>[16x]MVSLEKNDHLMLARQLPLKSVALILAGGRGTRLKDLTNKRAKPAVHFGGKFRIIDFALSNCINSGIRRMGVITQYQSHTLVQHIQRGWSFFNEEMNEFVDLLPAQQRMKGENWYRGTADAVTQNLDIIRRYKAEYVVILAGDHIYKQDYSRMLIDHVEKGARCTVACMPVPIEEASAFGVMAVDE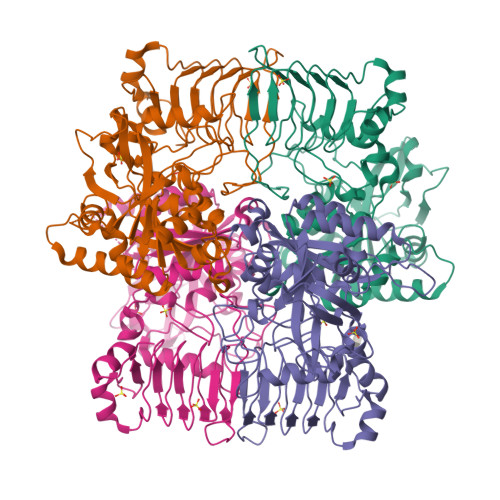NDKIIEFVEKPANPPSMPNDPSKSLASMGIYVFDADYLYELLEEDDRDENSSHDFGKDLIPKITEAGLAYAHPFPLSCVQSDPDAEPYWRDVGTLEAYWKANLDLASVVPELDMYDRNWPIRTYNESLPPAKFVQDRSGSHGMTLNSLVSGGCVISGSVVVQSVLFSRVRVNSFCNIDSAVLLPEVWVGRSCRLRRCVIDRACVIPEGMVIGENAEEDARRFYRSEEGIVLVTREMLRKLGHKQER>HMGSMALDGIRMPDGCYADGTWELSVHVTDLNRDVTLRVTGEVHIGGVMLKLVEKLDVKKDWSDHALWWEKKRTWLLKTHWTLDKCGIQADAKLQFTPQHKLLRLQLPNMKYVKVKVNFSDRVFKAVSDICKTFNIRHPEELSLLKKPRDPTKKKKKKLDDQSEDEALELEPGILAVSQPVTSPEILAKMFKPQALLDKAKTNQGWLDSSRSLMEQDVKENEALLLRFKYYSFFDLNPKYDAIRINQLYEQAKWALLLEEIECTEEEMMMFAALQYHINKLSIMTSENHLTTDVNPECLVSPRYLKKYKSKQITARILEAHQNVAQMSLIEAKMRFIQAWQSLPEFGITHFIARF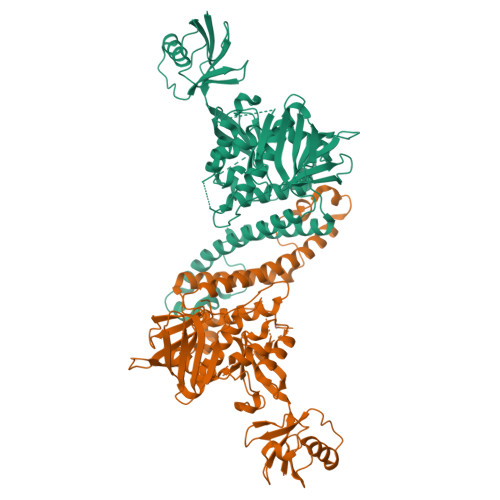QGGKREELIGIAYNRLIRMDASTGDAIKTWRFSNMKQWNVNWEIKMVTVEFADEVRLSFICTEVDCKVVHEFIGGYIFLSTRAKDQNESLDEEMFYKLTSGWVLVPRGSGSGSGSKSAVTTVVNPKYEGK[2x]> MAHHHHHHMLKLIVETKTLVQSLGFASSVVEKRNVIPEYANIKLSAKDGNLELSSTNMDLYLSQKIAVQVVSEGECTVSTKTLNDIVRKLPDSELTLTDLGTTGLEIKGKNCKFNLFTLPVSSFPAMDSINPEASFKISCTDFAKIIESTKFSISLDETRYNLNGVYLHIKDKEFCSAS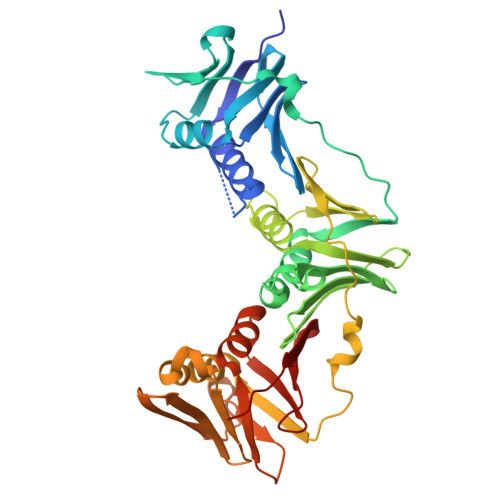TDGHRLSISWVTLEKQIKNFGVILPQKSAEEILKIVKDPKNINEDIEILLSSNKIKFICNENTSMLSKLIDGTFPDYSTFIPESSSSKLVINRKMFADSIERIAIITVEKFRAVKLSLSRETLEISAVGEARGNAKEVINSSQDKESFYEYNSDESLAIGFNPQYLEDVLKAVKSDVVELYFSDVSAPVLIKFPENPKDIFVVMPVKV>[6x]MAKNNAVAGFNALNGVELNLFTTDELKAIHYA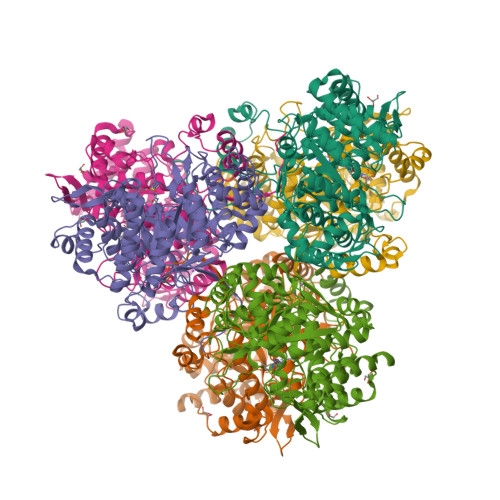TMEVLMDPGIQVSDPEARQIFKENGCEVNEKTNVVKIPEYLVRKALQLAPSRFVLWGRDKKFNTVQECGGKVHWTCFGTGVKVCKYQDGKYVTVDSVEKDIADIAKLCDWAENIDYFSLPVSARDIAGQGAQDVHETLTPLANTAKHFHHIDPVGENVEYYRDIVKAYYGGDEEEARKKPIFSMLLCPTSPLELSVNACQVIIKGARFGIPVNVLSMAMSGGSSPVYLAGTLVTHNAEVLSGIVLAQLTVPGAKVWYGSSTTTFDLKKGTAPVGSPELGLISAAVAKLAQFYGLPSYVAGSKSDAKVPDDQAGHEKTMTTLLPALAGANTIYGAGMLELGMTFSMEQLVIDNDIFSMVKKAMQGIPVSEETLAVESIQKVGIGNNFLALKQTRQLVDYPSNPMLLDRHMFGDWAAAGSKDLATVAHEKVEDVLKNHQVTPIDADIFKDMQAIVDKADKAFRGMGGHHHHHH> MANTKYNKKFLLYLAGFVDGDGSIIAQINPNQSSKFKHRLRLTFYVTQKTQRRWFLDKLVDEIGVGYVRDSGSVSQYVLSEIKPLHNFLTQLQPFLKLKQKQANLVLKIIEQLPSAKESPDKFLEVCTWVDQIAALNDSKTRKTTSETVRAVLDS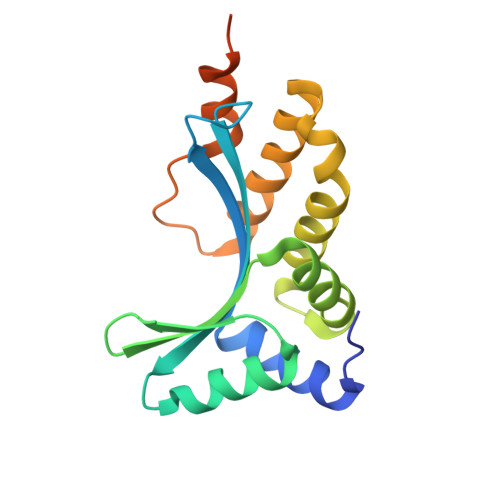LSGKKKSSPAADWSHPQFEK Ciliary motility is regulated by the conserved nexin-dynein regulatory complex (N-DRC), which links adjacent doublet microtubules and regulates and coordinates the activity of outer doublet complexes. The N-DRC is a large 1.5-MDa, ~50-nm-long Y-shaped complex with two main regions: the base plate and linker regions. The N-DRC bridges neighboring DMTs and restricts sliding motions between DMTs. Here, using cryo-electron microscopy in conjunction with biochemical cross-linking and integrative modeling, we localize 12 DRC subunits in the N-DRC structure of Tetrahymena thermophila.

We obtained the 96-nm repeating unit of the DMT at a global resolution of 3.6 Å, containing the N-DRC base plate. A high-resolution cryo-electron microscopy (cryo-EM) study of the DMT from C. reinhardtii revealed that DRC1, DRC2, and DRC4 form the core structure of the base plate. The main scaffold of the N-DRC comprises coiled-coiled proteins, including DRC1/2 and DRC4A/4B complexes, which start from the base plate and span through the proximal lobe of the linker. These components play a pivotal role in stabilizing the N-DRC and contribute to mechano-regulatory signal transmission. The role of DRC1, DRC2, and DRC4 proteins as the core structural components of the N-DRC agrees with earlier analyses of the N-DRC in C. reinhardtii (N-C-term tagging SNAP, BCCP)41 and biochemical studies. In accordance with our model and mass spectrometry analysis of different knockout DRC mutants, scaffold proteins should assemble onto the DMT first before the other N-DRC subunits dock onto the core scaffold proteins.

> MNPSQTQKGKIQIQVSRGSIDLLVRTMYEDINNIKLKNERFQKKKRAEDERRRRERYAEIQQEAIASGKKNAALEMKWAELKELDECEELNREMQDQQQTFQQIIEGKENLRKEFEEELKRKDDEYVKMLKEQSNDIKDMISKMRSQFYKIRDANMQELEDIERHFEQERSNLLNEFKAKIQATFKKHLDLEEQYVKEHAKTEEEQTKNIEDLRIKGAKHYAELKITMETEIQDLEKCFEDMKALYQLITEKLDYSLKVLQEKFHENNSMCDELKRKENNFKNRLKQLTKDYKQYDKKFKLENKNLTQEYKRIIRQFKELQKKFKHFEKADLDKYSEIQKMNEAEVKELKDKIIKCNITIHIQQLGMQWIPPQSEEEILAQQKLQLEQGGKAEEEEEREFEFCISEIKIGEICNIILEEADFLIDDKLREELEGSAEPEQIFQRLDCIKKCLYIDSEDEMNLFFRELITKCRVKSAEEIEEEARKQLLLLGLIKEAEENENPEGEEVQQQEGAQQKKKEEGNKKDDPKGKEGAKDSKENANPQGQNKSNQDERKKKKDGQDDHAGQGQGQYDSNQGGMGENQEEGENAEGQENLEGEIEKEIDLENTQINLNEVVKFLQNWQANKDKRKEKLEKESSKKAVKQETEREKKERIAREGKKYWEKLTQVLPERTFRIWNVNFFKFSFEKQILLNQINKLRFWTDLCPNIMNFFWTDKNQSKKPVNCITKMKNQRIFQINTYKLIMNLLSALQDSLIQIKDKDDFIQTKISTNLFTFHNFQILLQIFIVNQSFLFIRLCQSYSKKIILLIKNINQKLFNLSNFKNQFSF;> MALLGKTLKGRSTRPGGIPQKRNIKWRQLAKNQEEFDQLKQLAKMKREGLKARIKDEQKVVTFNKKKLITYWRKIMRIAKTEQLKNEIDIYSQNNQRELDSKEAFIQMLDKNLDEAEDQFQIALRNHLIHIENLMQLQEARMRGLAEEFNRDVNILETEFDLEREEMVKTHKTQLKELEDMIETVKEEDKKKTEEAQNEFSQFKEETKNKNLEETNVMKIILETKQTKYYTELEQMNSKFQSDTSNKVKDHQFYHAHNKNRKQEIDRYLRTISSKKAKIDLMKLKILQHCKEFNARNSALKKEKENISRNYHELKLKMQKFREEESRRLKELSNNSRNAVLKLREYCALGEKILKTAELCRRLETEKEKVLPFYESSVDEDQIPEQLKNEFEHLKKEDAEEYAYLNNFYKRYNKVLLDKLAIEKQKENLQRDNQLLKSLLKQYLDGISLNDDVLKNENNPLLVVNHKFNLGKMPVEKIENKTVIEGVFEVRNTSHQLQGQRAPPFQ;> MSKAAKAKKNVPVVSKLEADARKAAEGVNDNESEEFKKAMRKEARALVEQFNEEKKLLAFYQQERQKINYNWIIAKKELEDKKSELINKEREIQDLQENHFMTLNVYKQKIKHLLFQNQDQQSELKKDVEVTLKQLEDQHRIKSRELKTDVRSLKVTKKEQEISQQDYLFALKSEHDKQMTLMRQDYERQVNDIKRKYDLKMQNLTKEMEEARAAMIKQLEDNKNQKIAEIIKEHTQKYNDIKNYYSEITATNLDYRKTLKNEIKELQTKDEEYKKTLQQTEKGYKELNEPLQALGIEIIQLKKQDEEQEAIIKEKEELKQKIDNQERLFRKLEYEYEVKLQQFQYLERERNALYAKFNQTVFEIHQKSGLENLILEKKVTNLREDLEIKDLQIHQVLTAANIDPNSVGSINKSLEEVESLKNELISELQAQLKQIRKAHSHMVKAYEGKLSEFVIPVEELGFDPLVPTNTD;> MPPKKAKGKKKKEEEPDDEYKSMTGADLTQTLEKLKERVNEMRTNRNYIQMDRDMVENFYHNTLKEISEVKTKISNKETEAEEKESKHRIDVKVFLQKVKHLEYEQEKSNLNIEDDGKKAKEKEDAYFEDITKNMKQLKTQLKSEYLEKEKANIQQVQEEKKDHQSLLKIQQKKFDELINNLIIKYEERLAKLKEDLELKLKVEIHELEERKNLHINELMNNHEKAFAELKKYYNDITAENLNLIKAHKEKIAQIYANIQLNTKNVADNQAKNEQLKEPLAKHREIRNKLKEDLKQFAKHKMSLQNLKSKAITLKDKITKLERDGKDLDEKYEKVVREKQELEKKFEDITQEVKKNADLNNNVLSNRLQILLKEYNNKEEELRTIIDNAGLDHNLHEQLKQRVQQSIEAKNTLIKNLKYSIHHATKAYNDAIRVYEAKLVEFGIPIEELGFQPLETITSSMPAGLVSS;> MATTTNILHDVVRDQSMVNYVSNRDRPLYFKRPLVPQMTDIPLHISRPPVDQQVDYQTMQMQQNATIVEAPTKDAFVQTDYRESETQTDPYTPKCFVRDGDHPEVMELKDYKYGKGLPASIEELEQIELNREKVWFENSLPPISDEASFNLRRKLMEEQELREWSKKENEIKKFQNEKLYLLQQALIEREKEVEDKSQERIEEIRQQKTEHKNRQIAKIQRKKIKIDRKMTKSRKMQGKETLKRDIIEDYANFASRVYAGITHEGLSLDKIANKYEVQPLALGNYEMLQALHEGIRPREFETRVNLKKEIKEIEKNYTRLENYHRGELKKAQDEINGVHEQSKAQQKQEGNNFSYRNFENKIRPATPTWKYDTDFNISPSLITEIQEYRGPNGVQLMQAADKREEAVLLLQRLLRGRTTQNIMYEGKKKRTALIEELLTVAQIENLEEDKAEEVLMQQHEEKVKNAVLESIQGEVIAETMDELSKELLRIKQERKIQQMVEIAEKDRRIREIEEAGKRQAEEILRDREDVLHNQLIRVHQGTVDTYLDWLMSNALEQSSARQATIMTNLRKAKFNLPLEDFERKYNNNQTLIKDLVHSFLIPNVQRSKLKKQIQLEEKRFSEAAKRSLQQTITRASNKHANVQN;> MDQGEFIQDDNDQDYDQQEGDDENNDYMEDPQQDNNYNQNGDNLDDQGQDDDGGQNNLQQPSVPPEDDEDDDDDFPEYANEQNKRLNEIIKKKRKLIKDISAKIEEKSDRTKVLQEHLKNVEQELLHTQALIDAKNKEIETEDHMKQIAERQSGRIQSELKILEKRSIEQQEKLNDVQNQIFRGNEKMDQYKLEMNWNQEELEQWALAARQKEEDNLTLEKYKRADEVKIKELNLAIEKLTAEVGRKQNELEKEITETQAAQIELDKTAEEFKRQHEERHKLFLQWQEVTEIISKRDLAIREEGENFARIKIEIKSNKDALEERKRILKEAKEENKRIQMANELMERQNIQQISDNKHIEEQLAEKKADVEILKNQVSAFASDLSSKKNRIAILSQELLAKKQRLNAAQKKYQAHQVKLKNEEIMAKQYENDRSYAEEKYRKNEKEKKELEKEIRTQKENLFKHTQELFKHREREANLYGEIQGNMAACRNLQSHITKLNQEFQRQQELLYNAEYQIQLMERRVARAKGERTLEEKKDLENEIMNAERELGGVTGQNKELIESLKNLDDEIRTVKKKLAYVEEENTKYSSLIEELILENDMTYQDLNKIIKQKEEVLVQHDTMKLEIKKINESLNGATEKVFNLENQIYQLEMSMQEREKEIEVHKDVLMTEHKAAEEERHKIAVELAERKNKVKNLKIKYESLVQKNKASNGEVESVHEHSQAYYVIKAAQEREELQRKGDELNAKILKNEKELKALDNTLNHLKNRNSNYRDKFLNKGVTTQHREEAEGLEEQCRAASQNLFKKRDELQKLQKEQEEDTRRYTEIKNKLERLYEQHQSLDQEISKYQKDIDQQGDKLQRAQNSLQRNYQLAVNKNQNFINPKNPHMIQVKLDNQNNLYKTLLQGLYSLQQDIPELSSVVDEILKEQRIQNNKAPSSIDINSKRSSQSGRSQRSQRSNISNQ;> MSNQQGPEDNNLEDDMAYLPADHPLLAKLQIDLTKQLTDEHERVDQKLIEIDANLKKLEKTKEDIGVRLYSVQQQLAENQMNFEQAHENYNWVQKLRIEAEQKLKTESEVYDAKKKELEELRKKYLKAQDELSKLTRTLYQINEFNQQMKGQIINTKTNTYRAEENVVNLEAQKKKQDLLIDTMNEEIKRQTEQKTILTAQLISQKEETEQAKQILKEAHLEMQKIIASKKNLLERWQKSLMTMQRMDNALQAIKEALKGQQELNLQIGTELNGVNAEIRKETEIQESLEGKNKKFDYEKDYLQKKYNELQEEKSKLEAQINLLTQSLRQTETEAGRAEIDKRNIEDQMNLIETNIMKLHTETKKLWEDLVHQKSEHTTIEKTATNLNKQANQISIEIEDKSVELENLLNEIARVKIDQLNTLSQIEVLENKRREVIKEREEKEITVATYEVQIRQGHDLNEKKQHEVGRLNREHDKLSSVQSDMSRGPLEAKRNNLIRKTQELGKENDLMQREWIKKQTLLVTQNNRLNKIEEDVSQLKTKQTILEQKKLRLNNNYRIYEKDIREIQNALKNLRNEMNKLNDAIYRNKEKQQKLDNENFNIKSEFVEKLKELEKESVKLEVEIDRLKEEKADLLAEIVESERQILLWERKIQLEKEMQDALDPTVGQTEIQELKREIHRMELRLDDLRKKQEAIIAEMERAVYKRETIQLKYMNKDKTFSNSNSMSQKSSSISAASDNSAQITKKIAQLKTTLNQTTRNAEQMEKAIKNKKIELDDLNAQIEGNNDNLQKLESDCYNKNIELTKHKLERSTNILSISCMQNKAKKLEDLVAGKARLSVPEATLMTKYEELRDKNQEIKEALQKLCDDAPQYVEVLNYLIDLNVGDDDEDQEQ;> MASEDGEMPSQFEGIDPEQLTESQMQQYMMEMQRQGLLDSNMEGGQYEEGYEEGQEGEGYGEEYGDQDYDGNQNEYDSQQDSQQQGHDQVNEMHQDRYDRRVNSEISGNYEADDETLRKIRRDLLDNINLERRHRDLQPVYIDLTTNNISQYYSEYLVNNEHNQDFYENAKVRYNNLGECELCHITAKFEPDADITKEYIYDYFMEIGYLFLESEEEKRIILNPANNHIGIGVFFDEIQIVVVLILSEKVLCIQKISQPEQNKIEIRGKMLDENFGIYAIRIMNVDDQKKDIKGVGPEFIEYTRSTQEWMASFELELYNQDRMAIEYYTRVSPDSIPYKKKQSKNEKLTYKHLQLRLRTPFQIYPDPKYAAEDEKERIRKEQEILAHEEQERKEREENDAKRLKQSRKDYGDGQYDDDEHGQDDFNSQSDISDKDKHHDSMHAEQEQNQQAAQQQQDTISNKEIRQELEMAITEAQRQHDEFMLQNHKLQEEIKLLKNKNDGFVDRSNETAMNEHKYLNTLAHVHQIRLDLKQTQTRYNQMSQELQKKLEQKQKKCNEIKYAFLELKREVAKKAANSRTDKPIPEQQINEWEKAELQKSKELQELRLQILRLRNAYVKNQKILKKKEELAEGLHLIDFEQLKIENQTLNEKIEERNEELHKLKKKNTTTIQILTHTREKLGFVQGENGELNSQNVRKDQELDDMRKQLTQQKKTKDKLRSVNLTLKQQTGIVNSEELGQDYRDLRTRVSKLEEEKKRLEQKLRSMHEAIKTANQISTQNMQSQNNSLKKPYQPY;> MNQDKHPEITDEEQELITVEELSQKLELLYKDMEQIRRENLLFEAYLARNRKEIAKEDEVSEDKKGKGKKKDKNVDKKSLLLTNEEKFEIAQQEQDALKKQIDDGRIKSDQILETLRAILEETDMAITEIRKDAFDFQREILVGGENSRTGKIEAEKIIKFFEEKERQKDALIAKYSSKRTNLERQILKTNNQIQKKEEMGDDLKFIDFYQLQIENKKYVKEIDDKNKKLLALKISTNRISQTLKDEKQNLKQELDKGKEYASQMSERKKKISKIDAQIKSVKKVTSKLEKDRKIYDKQKEIFVQDNQDDVPQIMKYVQYKSKEQQLLYAIQNLERKIEIAELAYKKANRILQSSQQFQQK;> MFKNTFQSGFLSILYSIGSKPLQIWDKSIRNGHIKRITDQDILSSVLEIMGTNVSTNYITAPADPKETLGIKLPFLVMIIKNLKKYYTFEVQVLDDKNVRRRFRASNYQSTTRVKPFICTMPMRLDEGWNQIQFNLSDFTRRAYATNYIETLRVQIHANCRIRRIYFSDRLYSEEELPPEFKLFLPIQGQNKTNV N-(5-AMINO-5-CARBOXYPENTYL)GLUTAMIC ACID | 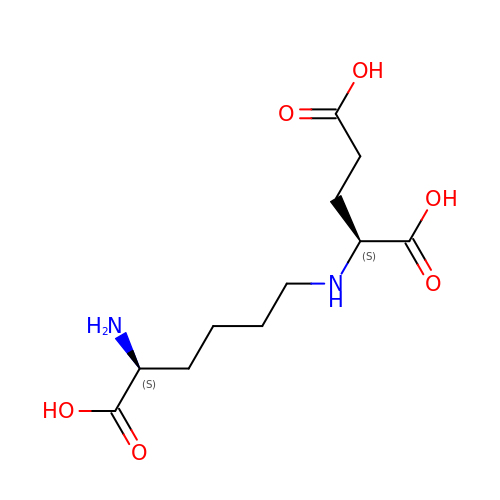C11 H20 N2 O6 | ZDGJAHTZVHVLOT-YUMQZZPRSA-N>GPASQTPTSDETIWDLSPYIKIFKDGRVERLHNSP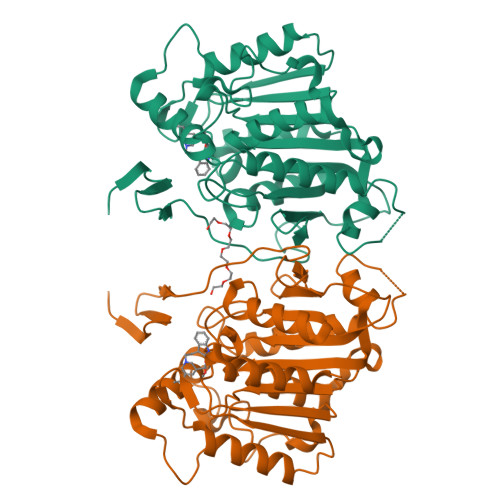YVPPSLNDPETGVSWKDVPISSQVSARVYIPKISDHEKLPIFVYVHGAGFCLESAFRSFFHTFVKHFVAETKVIGVSIEYRLAPEHLLPAAYEDCWEALQWVASHVGLDNSGLKTAIDKDPWIINYGDFDRLYLAGDSPGANIVHNTLIRAGKEKLKGGVKILGAILYYPYFIIPTSTKLSDDFEYNYTCYWKLAYPNAPGGMNNPMINPIAENAPDLAGYGCSRLLVTLVSMISTTPDETKDINAVYIEALEKSGWKGELEVADFDADYFELFTLETEMGKNMFRRLASFIKHE[8x]>MAIGEFMVSLPRMVYPQPKVLTPCRKDVLVVTPWLAPIVWEGTFNIDILNEQFRLQNTTIGLTVFAIKKYVAFLKLFLETAEKHFMVGHRVHYYVFTDQPAAVPRVTLGTGRQLSVLEVRAYKRWQDVSMRRMEMISDFCERRFLSEVDYLVCVDVDMEFRDHVGVEILTPLFGTLHPGFYGSSREAFTYERRPQSQAYIPKDEGDFYYGGAFFGGSVQEVQRLTRACHQAMMVDQANGIEAVWHDESHLNKYLLRHKPTKVLSPEYLWDQQLLGWPAVLRKLRFTAVPKNHQAVRNP[2x]

One important example is the biosynthesis of human ABO blood group antigens, which is the most important blood group system in transfusion and transplantation. GTA catalyzes the transfer of GalNAc from UDP-GalNAc to the H antigen acceptor (HAA) (α-l-Fuc-(1→2)-β-d-Gal-O-R, where R is glycolipid or glycoprotein) to form the A antigen, whereas GTB catalyzes the transfer of Gal from UDP-Gal to the HAA to form the B antigen. Among these is the enzyme AAGlyB, a dual-specificity GT, which can bind and utilize either UDP-Gal or UDP-GalNAc with equal efficiency. Each letter corresponds to one critical residue in increasing order such that the AAGlyB chimer would correspond to GTA-L266G/G268A.

The previous structure was obtained in the absence of acceptor, thus in the present study we soaked HAA acceptor into AAGlyB crystals together with 1 and Mn2+. The solved ternary structure shows well defined density for both HAA and 1 including the 5-substituent at the uracil base. Importantly, the entire active site loop in both chain A and B of the asymmetric unit as well as the C terminus of chain A are well resolved in the AAGlyB-1-HAA structure and in a conformation that has not previously been observed. However, in this new conformation, Trp-181 in the active site loop is not stacking to Arg-352 in the C terminus, as in the closed conformation with UDP and HAA, but to the formythienyl substituent of 1. Moreover, the C terminus of chain A has adopted an ordered state up until residue 353, which is folded over the donor binding site in a conformation alternative to that observed with the natural substrate. When comparing the AAGlyB-UDP-HAA complex with the AAGlyB-1-HAA complex, it can be seen that the C terminus in the latter structure fails to form the short α-helix, and neither His-348 nor Arg-352 interacts with the acceptor or the donor analogue. In this alternative conformation the main chain of Val-351 now forms two hydrogen bonds to the formylthienyl substituent of 1, and Asn-353 is forming hydrogen bonds to the backbone of residue Trp-181 as well as the side chain of Gln-182 in the internal loop. These additional molecular interactions provide, for the first time, a structural explanation for the tight binding of 1 to AAGlyB. The structure of the AAGlyB-1-HAA complex with a complete flexible loop and C terminus reveals, for the first time, a new, “pseudo-closed” conformation for this enzyme. Our results suggest that this pseudo-closed conformation allows the transfer of the sugar, albeit at a slower rate than the native, closed conformation, and could therefore be the reason for the small, residual turnover observed for AAGlyB toward 1.> X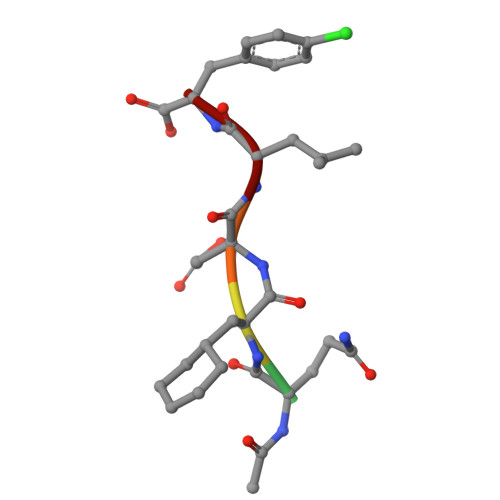QADLF> MTAPLPEGLTPDAVDTLTELSAIIKKLRAAQQQQAANPSSQ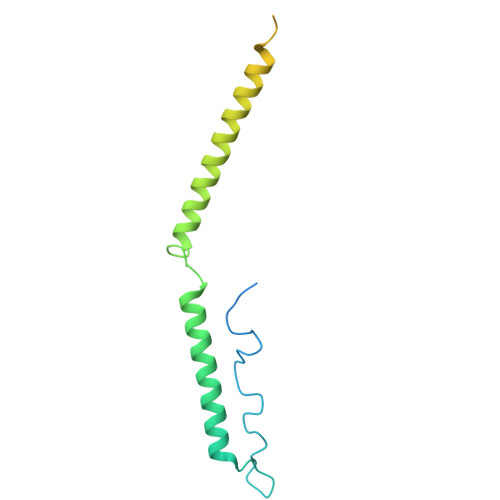AAAGGPGTTGAPGSQPSSSGPNATAAGGAIGTTSLPSSATTGPTPSNALHSVKELPATTDPIKHKLQRARAAVRLLGDMSRTMAQQEAELARLEERRRKQAAMLAKAQEEGARLSKGFGEVGETPVVLVETGDKMAME>DDAAIQQTLAKMGIKSSDIQPAPVAGMKTVLTNSGVLYITDDGKHIIQGPMYDVSGTAPVNVTNKMLLKQLNALEKEMIVYKAPQEKHVITVFTDITCGYCHKLHEQMADYNALGITVRYLAFPRQGLDSDAEKEMKAIWCAKDKNKAFDDVMAG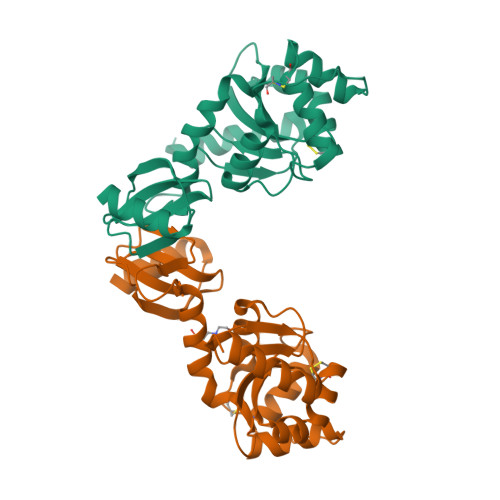KSVAPASCDVDIADHYALGVQLGVSGTPAVVLSNGTLVPGYQPPKEMKEFLDEHQKMTSGK[2x]>[2x]QGPPSPGYYPSSQITSLGFDQGYTNLWGPQHQRVDQGSLTIWLDSTSGSGFKSINRYRSGYFGANIKLQSGYTAGVITSFYLSNNQDYPGKHDEIDIEFLGTIPGKPYTLQTNVFIEGSGDYNIIGRELRIHLWFDPTQDYHNYAIYWTPSEIIFFVDDVPI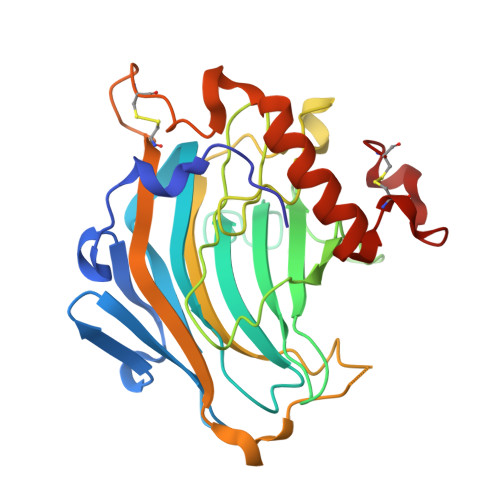RRYPRKSDATFPLRPMWVYGSVWDASSWATENGKYKADYRYQPFVGKYEDFKLGSCTVEAASSCNPASVSPYGQLSQQQVAAMEWVQKNYMVYNYCDDPTRDHTLTPEC> MSGIVIDKEKVHSKMPDVVKNAKIALIDSALEIKKTEIEAKVQISDPSKIQDFLNQETNTFKQMVEKIKKSGANVVLCQKGIDDVAQHY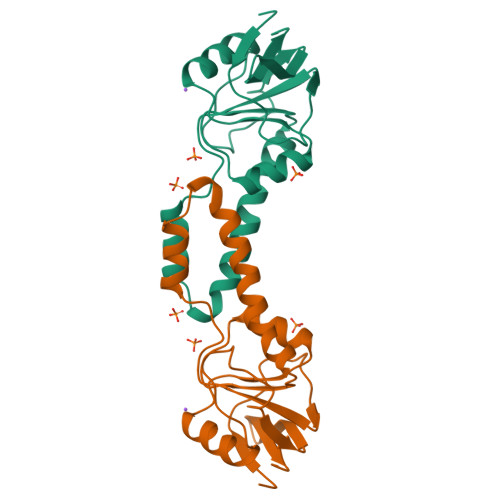LAKEGIYAVRRVKKSDMEKLAKATGAKIVTDLDDLTPSVLGEAETVEERKIGDDRMTFVMGCKNHHHHHH>MASMTGGQQMGRDQAGITGTWYNQLGSTFIVTAGADGALTGTYESAVGNAESRYVLTGRYDSAPATDGSGTALGWTVAWKNNYRNAHSAT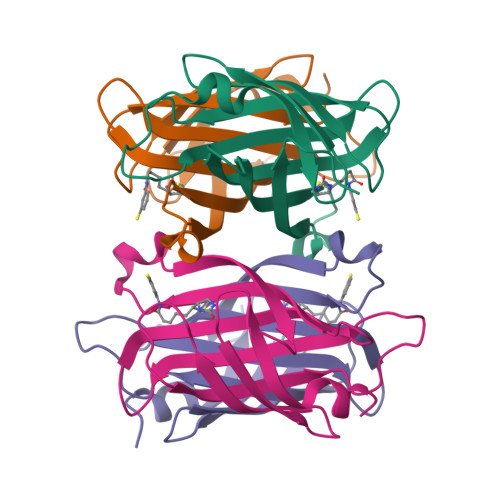TWSGQYVGGAEARINTQWLLTSGTTEANAWWSTLVGHDTFTKVKPSAASIDAAKKAGVNNGNPLDAVQQ[4x]> GSGMALSKSMHARNRYKDKPPDFAYLASKYPDFKQHVQINLNGRVSLNFKDPEAVRALTCTLLREDFGLSIDIPLERLIPTVPLRLNYIHWVEDLIGHQDSDKSTLRRGIDIGTGASCIYPLL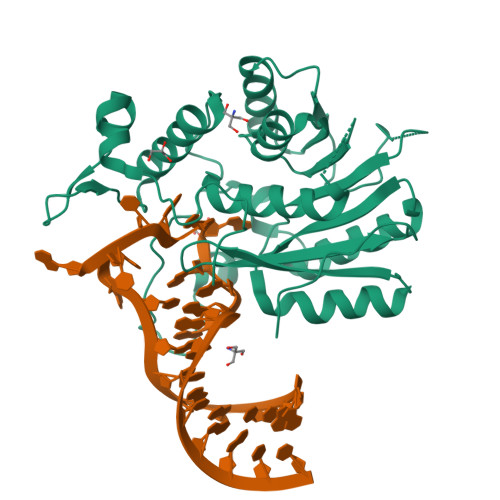GATLNGWYFLATEVDDMCFNYAKKNVEQNNLSDLIKVVKVPQKTLLMDALKEESEIIYDFCMCNPPFFANQLEAKGVNSRNPRRPPPSSVNTGGITEIMAEGGELEFVKRIIHDSLQLKKRLRWYSCMLGKKCSLAPLKEELRIQGVPKVTYTEFCQGRTMRWALAWSFYDDVTVPSPPSKRRKLEKPRK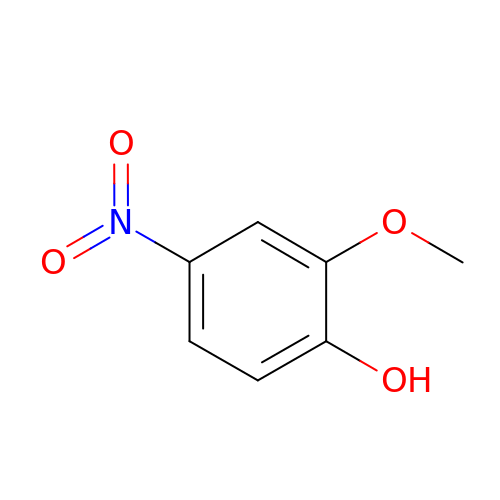2-methoxy-4-nitrophenol | C7 H7 N O4 | IZLVFLOBTPURLP-UHFFFAOYSA-N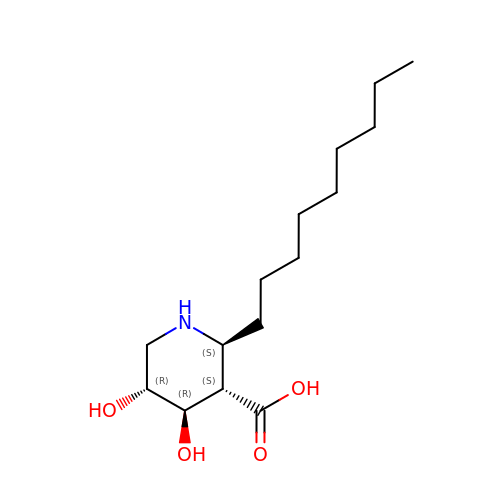(2~{S},3~{S},4~{R},5~{R})-2-nonyl-4,5-bis(oxidanyl)piperidine-3-carboxylic acid | C15 H29 N O4 | PFGVLKMJAGVUAN-CRWXNKLISA-N>[3x]MGHHHHHHHHMKFDNDSEKQVFDKLKKAIPGIIKEKCAGYDELYGYKLNPEGLTQEEVDKYYDEKIADRLTYKLCKAYQFEYSTIVQNLIDILNWRREFNPLSCAYKEVHNTELQNVGILTFDANGDANKKAVTWNLYGQLVKKKELFQNVDKFVRYRIGLMEKGLSLLDFTSSDNNYMTQVHDYKGVSVWRMDSDIKNCSKTVIGIFQKYYPELLYAKYFVNVPTVFGWVYDLIKKFVDETTRKKFVVLTDGSKLGQYLKDCPYEGYGGKDKKNNLTKQNVTNVHPTEYGLYILQKQIIEDVE

We report Sfh5 is a novel penta-coordinate high spin Fe3+ heme-binding protein conserved across the fungal kingdom that exhibits unusual heme-binding properties. As such, Sfh5 is the founding member of a new and conserved class of fungal hemoproteins, and provides the first demonstration that the spectrum of ligands for PITP-like proteins extends beyond lipids. In contrast to the known priming lipids of other Sec14-like PITPs, heme is not an exchangeable ligand for Sfh5, and the feeble PtdIns-exchange activity of Sfh5 is strongly enhanced in heme-binding mutants – indicating Sfh5 is not designed to function as a bona fide PITP in vivo. While the biological functions of Sfh5 remain to be determined, chemogenomic analyses forecast Sfh5 plays a role in organic oxidant-induced stress responses.

The crystal asymmetric unit (ASU) contained three molecules of Sfh5 with a single heme-Fe bound to each of the chains. Sfh5 adopted a typical Sec14-fold comprised of eight α-helices, five β-strands, five short 310 helices and a β-hairpin turn. By contrast, the Sfh5 helical gate was shifted by ~18 Å across the cavity opening relative to the position of this substructure in Sec14 -- thereby describing a ‘closed’ Sfh5 conformer. Again, in a strategy conserved across the Sec14-like PITP family, Sfh5 residue F228, located at the C-terminus of the KKFV gating element (KPFL in Sec14 and Sfh1), engaged K192 of the adjacent helix A6 in a cation-π interaction to stabilize the closed conformer. Only ~8 Å2 of the heme surface area was solvent exposed -- as opposed to 835 Å2 for free heme. In that configuration, heme b exhibited twenty-five van der Waals interactions with amino acid side chains of the residues that line the cavity, including residues F138, F144, V178, I187, I195, F211, V212, F218, I225, V229, and F237. Bound heme-Fe was in close proximity (2.3 Å) to the hydroxyl group of residue Y175, and tyrosine coordination was consistent with the results of safranin T dye-reduction assays which estimated an unusually low thermodynamic reduction potential for Sfh5 heme (−330 ± 3 mV vs normal hydrogen electrode). The Y175 hydroxyl group also engaged the Nε2-tautomer of the proximal H173 via a hydrogen bond interaction. Only two amino acid side chains (S191 and I225) reside within a 5 Å radius on the distal side of the Fe -- reporting the absence of a sixth coordinating ligand and establishing that bound Fe is penta-coordinate. That vacant coordination site on the distal side of the Fe represents a candidate substrate binding pocket positioned close to the Sfh5 protein surface and to which access from solvent is occluded by the side chains of K188 and K192 of helix A6 on one side and residues L224, I225 of helix A7 and F228 on the loop connecting helix A7 and 310-helix T4, on the other.>[5x]MAGGGDLDASDY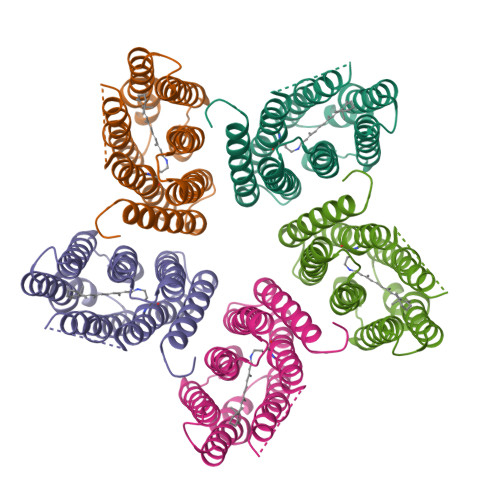TGVSFWLVTAALLASTVFFFVERDRVSAKWKTSLTVSGLVTGIAFWHYMYMRGVWIETGDSPTVFRYIDWLLTVPLLICEFYLILAAATNVAGSLFKKLLVGSLVMLVFGYMGEAGIMAAWPAFIIGCLAWVYMIYELWAGEGKSACNTASPAVQSAYNTMMYIIIFGWAIYPVGYFTGYLMGDGGSALNLNLIYNLADFVNKILFGLIIWNVAVKESSNA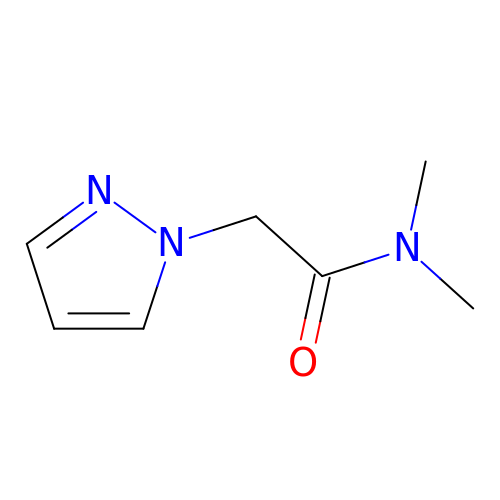N,N-dimethyl-2-(1H-pyrazol-1-yl)acetamide | C7 H11 N3 O | HTIDWWCOZGRQRN-UHFFFAOYSA-N>[2x]MYAYNGKLLDVDLTREKVKEVELSEDVLKKFYGGRGLGTYILWK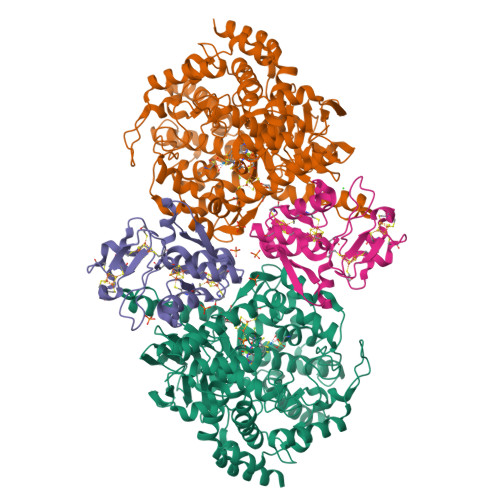ELGEKWEKVDPLGEENLLLILTGPLTGYYPGMKTSIVSKSPESNGVVGSVLSSELGLELKAAGYDGIIIRGKAKSPVYLFIHNDTVEIRDATKYWGMGGIELYKTLLKEVHEEIRKKEKLKGVPKEPAMIYIGKGGENKVRFAAIMTKLMHAAGYGGYGAVMGSKNLKAVIAKGSGPLPEVYDKEKMKVLLREFWKELFSMTTFREWGTGAGGYSVGHDRSSEPIRNWQEEYHDNEEISVVNFENRTWIKKYWADYGCPVNCMKISYLRYGPYKGSISDAPDYELQAYMGTNLGIFEPEKIVYLSYLVDELGLDGINTGNILGFAAELYQRGILTKEDLGFELNWGDEKAFAKLLHLIVEKEGIGKILAEGTYRAALKISEIKGIDVTKYAVHVKGIAVGAHGIRSELDYTKDISYAVSVQGGDHTSTAALPAKGYTGELVEAFYDSAVICNFVTKPGFEKIIEFGNALSGFNITPEQWLNEIGLRIIHLQRILLLLGGPDVYWDPRKDDDNPPRFYEPLPSGPVKGKAPNREDIKAKVKQYYEEIGYDEHGIPKEEVLEELGIGEAKREVKRIKKRLN;>[2x]MSEEVQERIWILITPDKCSGCRLCEVTCSLEHEGIIWPEASRIRVFELFPGINVPHTCVQCPDYPCVNACPTNALSVDEKTGAVVVNEEKCITCGACVLACPGKVPRIPAGKGSVVICDLCGGNPKCVEICHEAGHDALKIVTGNYRPIYRTFAKDPQEKSLDIARKVFGEDF>[4x]MSISASEARQRLFPLIEQVNTDHQPVRITSRAGDAVLMSADDYDAWQETV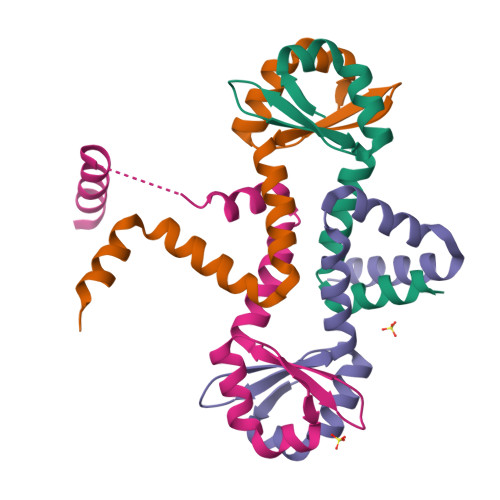YLLRSPENARRLMEAVARDKAGHSAFTKSVDELREMAGGEE>[2x]PLGSMKDYDELLKYY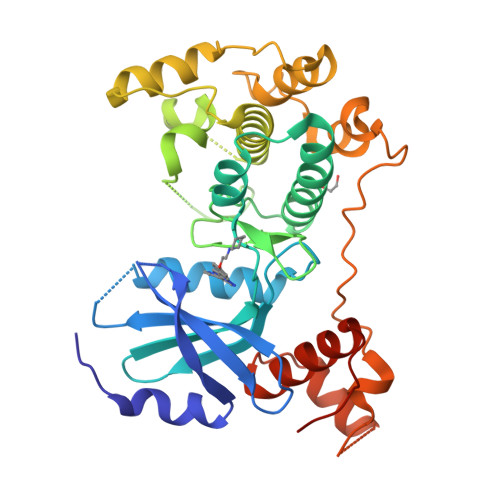ELHETIGTGGFAKVKLACHILTGEMVAIKIMDKNTLGSDLPRIKTEIEALKNLRHQHICQLYHVLETANKIFMVLEYCPGGELFDYIISQDRLSEEETRVVFRQIVSAVAYVHSQGYAHRDLKPENLLFDEYHKLKLIDFGLCAKPKGNKDYHLQTCCGSLAYAAPELIQGKSYLGSEADVWSMGILLYVLMCGFLPFDDDNVMALYKKIMRGKYDVPKWLSPSSILLLQQMLQVDPKKRISMKNLLNHPWIMQDYNYPVEWQSKNPFIHLDDDCVTELSVHHRNNRQTMEDLISLWQYDHLTATYLLLLAKKARGKPVRLRLSSFSCG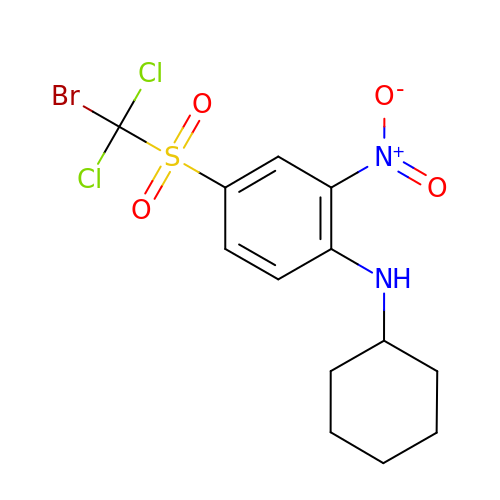4-[bromo(dichloro)methanesulfonyl]-N-cyclohexyl-2-nitroaniline | C13 H15 Br Cl2 N2 O4 S | REBZZEDLLSTDTN-UHFFFAOYSA-N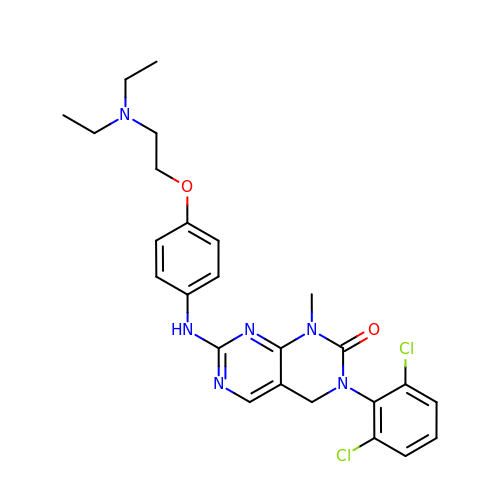3-(2,6-dichlorophenyl)-7-({4-[2-(diethylamino)ethoxy]phenyl}amino)-1-methyl-3,4-dihydropyrimido[4,5-d]pyrimidin-2(1H)-one | C25 H28 Cl2 N6 O2 | LQYPBKQMDVWUGO-UHFFFAOYSA-N>MAVERTLIIVKPDAMEKGALGKILDRFIQEGFQIKALKMFRFTPEKAGEFYYVHRERPFFQELVEFMSSGPVVAAVLEGEDAIKRVREIIGPTDSEEARKVAPNSIRAQFGTDKGKNAIHASDSPESAQYEICFIF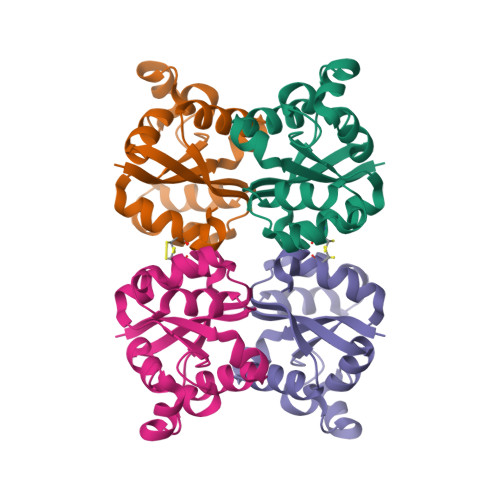SGLEIV[12x]>SMIAAYQARCQARVDAALDALFVAPREELQRLYEAMRYSVMNGGKRVRPLLAYAACEALGGAPQRADAAACAVELIHAYSLVHDDLPAMDDDDLRRGQPTTHRAFDEATAILAADGLQALAFEVLADTRRNPQEHAVCLEMLTRLARAAGSAGMVGGQAIDLGSVGVALDQAALEVMHRHKTGALIEASVRLGALAS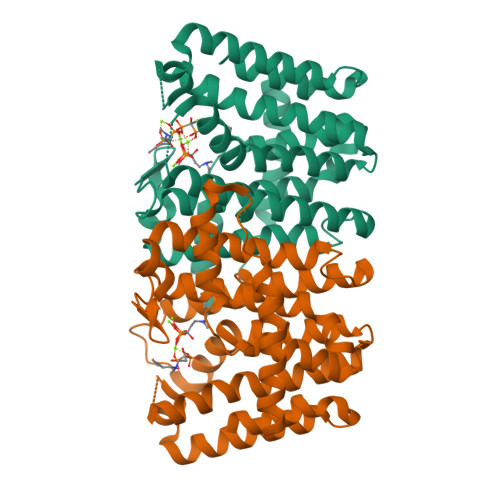GRAEPASLAALERYAEAIGLAFQVQDDILDVESDTATLGKTQGKDQAHNKPTYPALLGLEAAKGYALELRDLALAALDGFPPSADPLRQLARYIVERRN[2x]>[2x]ATAVNGAPRDAALWSSHEQMLAQPLKDSDAEVYDIIKKESNRQRVGLELIASENFASRAVLEALGSCLNNKYSQGYPGQRYYGGTEHIDELETLCQKRALQAYGLDPQCWGVNVQPYSGSPANFAVYTALVEPHGRIMGLDLPDGGHLTHGFMTDKKKISATSIFFESMAYKVNPDTGYIDYDRLEENARLFHPKLIIAGTSCYSRNLDYGRLRKIADENGA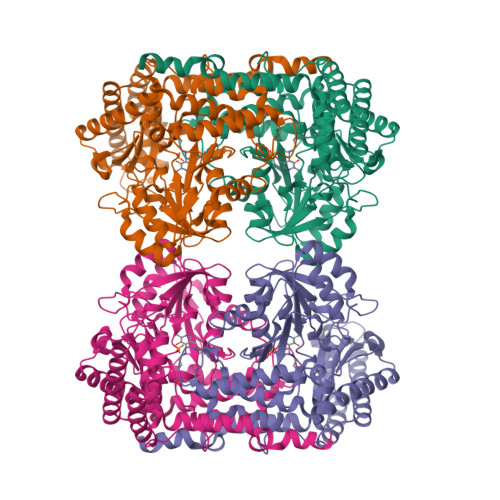YLMADMAHISGLVVAGVVPSPFEHCHVVTTTTHKTLRGCRAGMIFYRRGVRSVDPKTGKEILYNLESLINSAVFPGLQGGPHNHAIAGVAVALKQAMTPEFKEYQRQVVANCRALSAALVELGYKIVTGGSDNHLILVDLRSKGTDGGRAEKVLEACSIACNKNTCPGDKSALRPSGLRLGTPALTSRGLLEKDFQKVAHFIHRGIELTVQIQDDTGPRATLKEFKEKLAGDEKHQRAVRALRQEVESFAALFPLPGLPGF>MIAELFTNNALNLVIIFGSCAALILMSFWFRRGNRKRKGFLFHAVQFLIYTIIISAVGSIINYVIENYKLKFITPGVIDFICTSLIAVILTIKLFLLINQFEKQQIKKGRDITSARIMSRIIKITIIVVLVLLYGEHFGMSLSGLLTFGGIGGLAVGMAGKDILSNFFSGIMLYFDRPFSIGDWIRSPDRNIEGTVAEIGWRITKITTFDNRPLYVPNSLFSSISVENPGRMTNRRITTTIGLRYEDAAKVGVIVEAVREMLKNHPAIDQRQTLLVYF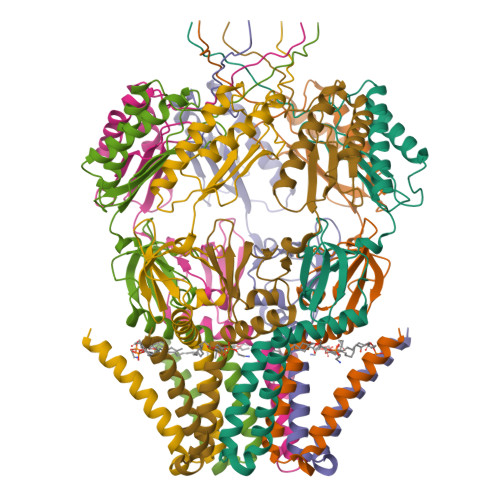NQFADSSLNIMVYCFTKTTVWAEWLAAQQDVYLKIIDIVQSHGADFAFPSQTLYMDNITPPEQGR[7x]> MRGSHHHHHHGSAEPPNMPSMAPVLKNIMPAIVNVAVQGYLPNDVTPPGSAGNDEENQPNNRPPQSRMPEKGRKFESIGSGVIIDPNNGVIITNDH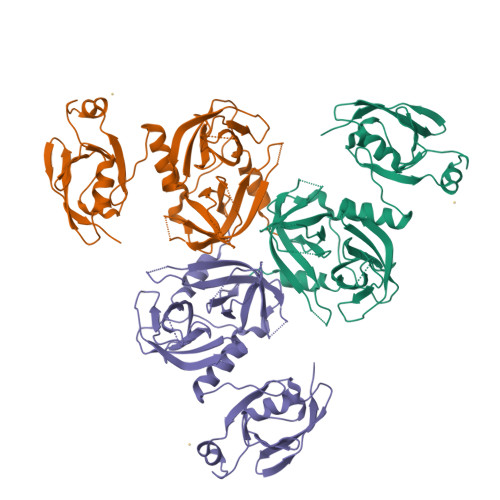VIRNASLITVTLQDGRRLKARLIGGDSETDLAVLKIDAKNLKSLVIGDSDKLEVGDFVVAIGNPFGLNSFGNSQSATFGIVSALKRSDLNIEGVENFIQTDAAINPGNSGGALVNAKGELIGINTAILSPYGGNVGIGFAIPINMVKDVAQQIIKFGSIHRGLMGIFVQHLTPELAQAMGYPEDFQGALVSQVNPNSPAELAGLKAGDIITQINDTKITQATQVKTTISLLRVGSTVKIIVERDNKPLTLSAVVTDIK> 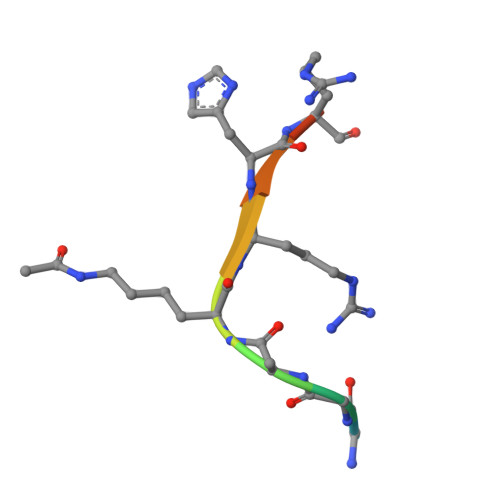KGGAKRHRKI> SSGQISIQPTFSVQR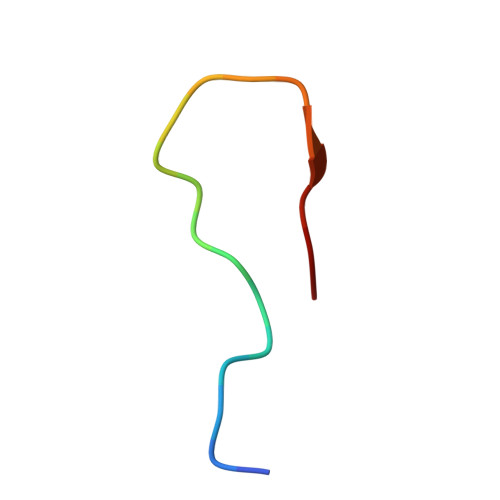NLPF>MLSIKDLHVSVEDKAILRGLSLDVHPGEVHAIMGPNGSGKSTLSATLAGREDYEVTGGTVEFKGKDLLALSPEDRAGEGIFMAFQYPVEIPGVSNQFFLQTALNAVRSYRGQETLDRFDFQDLMEEKIALLKMPEDLLTRSVNVGFSGGEKKRND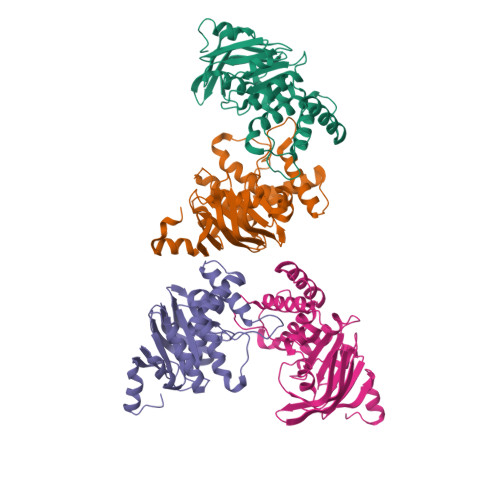ILQMAVLEPELCILDESDSGLDIDALKVVADGVNSLRDGKRSFIIVTHYQRILDYIKPDYVHVLYQGRIVKSGDFTLVKQLEEQGYGWLTEQQ[4x]> PSLLVLTFSPCVLLGWALLAGGTGGGGVGGGGGGAGIGGGRQEREALPPQKIEVLVLLPQDDSYLFSLTRVRPAIEYALRSVEGNGTGRRLLPPGTRFQVAYEDSDCGNRALFSLVDRVAAARGAKPDLILGPVCEYAAAPVARLASHWDLPMLSAGALAAGFQHKDSEYSHLTRVAPAYAKMGEMMLALFRHHHWSRAALVYSDDKLERNCYFTLEGVH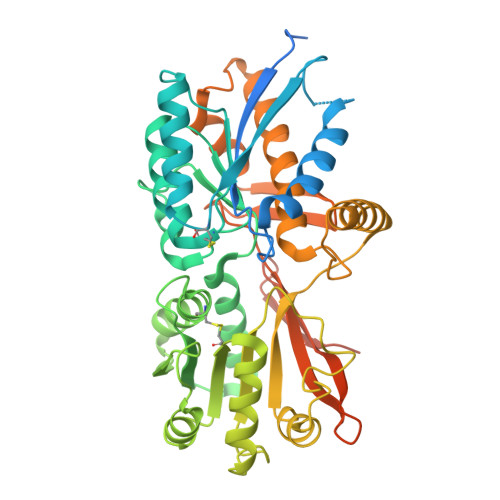EVFQEEGLHTSIYSFDETKDLDLEDIVRNIQASERVVIMCASSDTIRSIMLVAHRHGMTSGDYAFFNIELFNSSSYGDGSWKRGDKHDFEAKQAYSSLQTVTLLRTVKPEFEKFSMEVKSSVEKQGLNMEDYVNMFVEGFHDAILLYVLALHEVLRAGYSKKDGGKIIQQTWNRTFEGIAGQVSIDANGDRYGDFSVIAMTDVEAGTQEVIGDYFGKEGRFEMRPNVKYPWGPLKLRIDENRIVEHTNSSPCKSSGGLE>[40x]GGTDPATMVNNICTFILGPFGQSLAVLGIVAIGISWMFGRASLGLVAGVVGGIVIMFGASFLGKTLTGG

Here, we determine atomic structures by cryo-electron microscopy of three conjugative pili, two from hyperthermophilic archaea (Aeropyrum pernix and Pyrobaculum calidifontis) and one encoded by the Ti plasmid of the bacterium Agrobacterium tumefaciens, and show that the archaeal pili are homologous to bacterial mating pili. With structures for four bacterial conjugation pili (pED208, F, pKpQIL, and pTiC58 from A. tumefaciens) and two archaeal ones (A. pernix and P. calidifontis), it is clear that there is a common architecture for all and obvious homology, despite negligible sequence similarity. Each prokaryotic pilin subunit consists of two or three hydrophobic α-helices, with kinks appearing in some of the helices, such as in A. pernix and A. tumefaciens. Hence, pore diameters of all prokaryotic conjugative pili are sufficiently wide for the passage of ssDNA, but not dsDNA.

To extend the comparison between the archaeal mating pili and the existing structures of bacterial ones, we used cryo-EM to solve the structure of the A. tumefaciens T-pilus encoded by the pTiC58 plasmid to 3.5 Å resolution. The T-pilus has a fivefold rotational symmetry with a rise of 13.7 Å and a twist of 32.5° per subunit. The 3.5 Å resolution of the T-pilus map allowed for unambiguous model building and interpretation of the protein subunit, VirB2. The atomic model of VirB2 shows clear structural homology to the TraA subunit of the F-pilus. One clear difference between VirB2 on the one hand, and TraA of pED208 on the other, is that there are kinks in helix 1 and 3 of the VirB2 subunit, produced by Pro23 and Phe61, respectively. Similar to other bacterial conjugation pili, there is a stoichiometry of one lipid molecule to each protein subunit. The same analysis applied to VirB2 T-pili revealed a strikingly different set of PLA2-resistant lipids, with >65% of the phospholipids being phosphatidyl-ethanolamine (PE). The electrostatic surface for the lumen of the T-pilus generated by the atomic model is overall quite positive. While the lumen of other bacterial mating pili may have evolved to be optimal for DNA transport, the lumen of the T-pilus, also used for the transport of a diverse range of other substrates, has a positive electrostatic potential that would still allow DNA transfer, but not be optimal due to the greater friction resulting from DNA sticking to the walls. Surprisingly, the cryo-EM structure of VirB2 reveals no cyclization of the pilin.> GEESRNTTVLDTTTTLQSSGFGRAFFGEAFNDLKTLMRRYQLYGQLLLSVTTDKDIDHCMFTFPCLPQGLALDIGSAGSPHEIFNRCRDGIIPLIASGYRFYRGDLRYKIVFPSNVNSNIWVQHRPDRRLEGWSAAKIVNCDAVSTGQGVYNHGYASHIQITRVNNVIELEVPFYNATCYNYLQAFNASSAASSYAVSLGEISVGFVNKPVTIYYSIGDGMQFSQWVGYQPMMILDQLPAPVV;> MDNPNPGPDGEGEVELEKDSNVVLTTQRDPSTSIPAPVSVKWSRWTSNDVVDDYATITSRWYQIAEFVWSKDDPFDKELARLILPRALLSSIEANSDAICDVPNTIPFKVHAYWRGDMEVRVQINSNKFQVGQLQATWYYSDHENLNISSKRSVYGFSQMDHALISASASNEAKLVIPFKHVYPFLPTRIVPDWTTGILDMGALNIRVIAPLRMSATGPTTCNVVVFIKLNNSEFTGTSSGKFYASQIRA;> NPSYQQSPRHFVPTGMHSLALGTNLVEPLHALRLDAAGTTQHPVGCAPDEDMTVSSIASRYGLIRRVQWKKDHAKGSLLLQLDADPFVEQRIEGTNPISLYWFAPVGVVSSMFMQWRGSLEYRFDIIASQFHTGRLIVGYVPGLTASLQLQ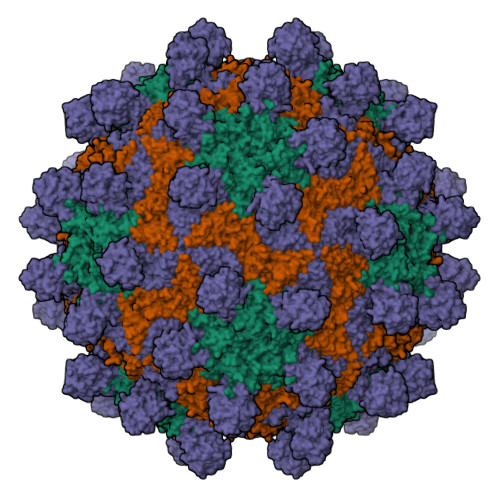MDYMKLKSSSYVVFDLQESNSFTFEVPYVSYRPWWVRKYGGNYLPSSTDAPSTLFMYVQVPLIPMEAVSDTIDINVYVRGGSSFEVCVPVQPSLGLNWNTDFILRNDEEYRAKTGYAPYYAGVWHSFNNSNSLVFRWGSASDQIAQWPTISVPRGELAFLRIKDGKQAAVGTQPWRTMVVWPSGHGYNIGIPTYNAERARQLAQHLYGGGSLTDEKAKQLFVPANQQGPGKVSNGNPVWEVMRAPL> GSHMTRTRMENELIVSKNMQNIIIAGNGPSLKNINYKRLPREYDVFRCNQFYFEDKYYLGKKIKAVFFNPGV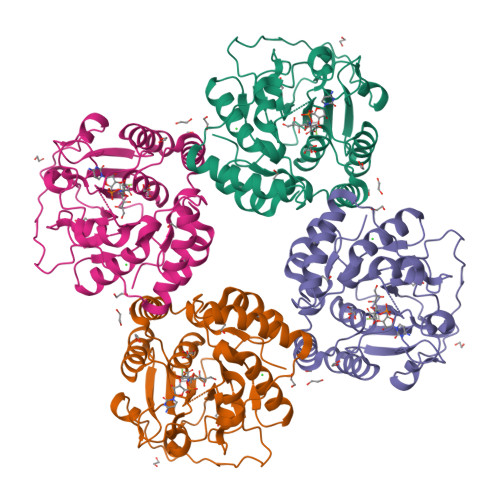FLQQYHTAKQLILKNEYEIKNIFCSTFNLPFIESNDFLHQFYNFFPDAKLGYEVIENLKEFYAYIKYNEIYFNKRITSGVYMCAIAIALGYKTIYLCGIDFYEGDVIYPFEAMSTNIKTIFPGIKDFKPSNCHSKEYDIEALKLLKSIYKVNIYALCDDSILANHFPLSININNNFTLENKHNNSINDILLTDNTPGVSFYKNQLKADNKIMLNFY(5R)-2-amino-5-[4-(difluoromethoxy)phenyl]-5-[4-fluoro-3-(5-fluoropent-1-yn-1-yl)phenyl]-3-methyl-3,5-dihydro-4H-imidazol-4-one | C22 H19 F4 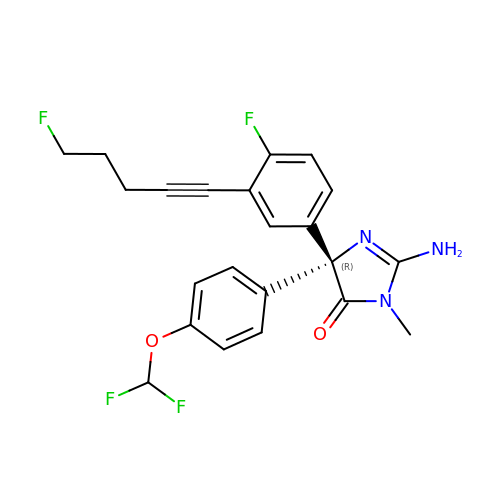N3 O2 | ZSIZOKHLIKKQIV-JOCHJYFZSA-N>GPGHMPEYQAQGLAMYLQENGIDCPKCKFSYALARGGCMHFHCTQCRHQFCSGCYNAFYAKNKCPEPNCRVKKSLHGHHPRDCLFYLRDWTALRLQKLLQDNNVMFNTEPPAGARAVPGGGCRVIEQKEVPNGLRDEACGKETPAGYAGLCQAHYKEYLVSLINAHSLDPATLYEVEELETATERYLHVRPQPLAGEDPPAYQARLLQKLTEEVPLGQSIPRRRK[6x]

The ubiquitin system, composed of ubiquitin-activating enzyme (E1), ubiquitin-conjugating enzyme (E2), and ubiquitin ligase (E3), regulates numerous cellular functions through the generation of various ubiquitin chains in a system referred to as the ubiquitin code. HOIP, as well as HOIL-1L, belongs to the RBR-type E3 family, and the family E3s reportedly generate polyubiquitin chains through a RING-HECT-hybrid reaction. Among them, HOIP contains the E3 active site. The linear ubiquitin chain functions as a scaffold to recruit other IκB kinase (IKK) molecules, and the recruited IKK molecules are then activated by a trans-phosphorylation mechanism, leading to the activation of the NF-κB signaling pathway.

Furthermore, we developed seven derivatives of HOIPIN-1, and found that HOIPIN-8 is the most potent LUBAC inhibitor among them. HOIPINs are covalently attached to the catalytic Cys885 of HOIP via Michael addition. The benzoate moiety of HOIPINs is the key element for binding to HOIP. The carboxyl group of the benzoate hydrogen bonds with Arg935, and the aromatic ring of the benzoate hydrophobically interacts with Phe905, Leu922, and the aliphatic portion of His887. The aromatic ring of the methoxyphenyl moiety of HOIPIN-1 and the 2,6-difluorophenyl moiety of HOIPIN-8 stack on the carboxyl group of the benzoate moiety and the guanidino group of Arg935, respectively. Furthermore, the two pyrazol moieties of HOIPIN-8 form additional interactions with HOIP that enhance the affinity. Thus, the 1H-pyrazol-4-yl at the 4-position of the 2,6-difluorophenyl moiety forms a hydrogen bond with Asp936, and the 1-methyl-1H-pyrazol-4-yl at the 4-position of the benzoate moiety is accommodated in the hydrophobic pocket formed by Phe905 and Leu922, and stacks on His887. The benzoate, 2,6-difluorophenyl, and 1H-pyrazol-4-yl moieties of HOIPIN-8 interact with Arg935 and Asp936, which are located in the LDD domain of HOIP. Arg935 and Asp936 in the LDD domain reportedly interact with Glu16 and Thr14 in the acceptor ubiquitin, and the Ala mutations of these residues abrogated the linear ubiquitination activity. Thus, HOIPIN-8 not only interacts with the active Cys885 but also masks the critical residues for acceptor ubiquitin-binding.>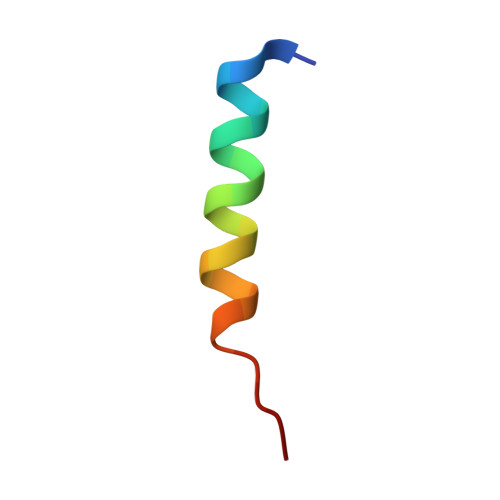 PELDDILYHVKGMQRIVNQWSEK> GIEDLIDTAIKNALRVSQPPSTQSTEATSGVNSQEVPALTAVETGASGQAIPSDVVETRHVVNYKTRSESCLESFFGRAACVTILSLTNSSKSGEEKKHFNIWNITYTDTVQLRRKLEFFTYSRFDLEMTFVF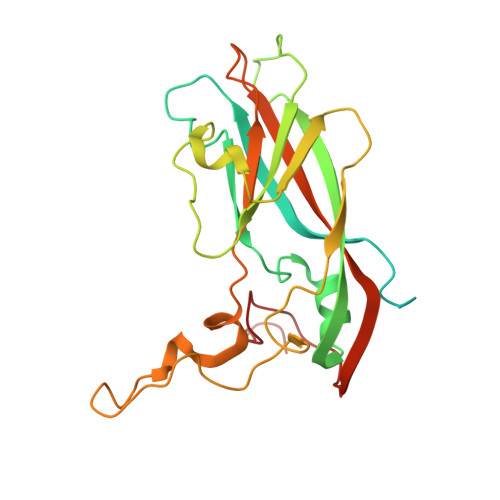TENYPSTASGEVRNQVYQIMYIPPGAPRPSSWDDYTWQSSSNPSIFYMYGNAPPRMSIPYVGIANAYSHFYDGFARVPLEGENTDAGDTFYGLVSINDFGVLAVRAVNRSNPHTIHTSVRVYMKPKHIRCWCPRPPRAVLYRGEGVDMISSAI> GPLGSPEFMEPLKVEKFATANRGNGLRAVTPLRPGELLFRSDPLAYTVCKGSRGVVCDRCLLGKEKLMRCSQCRVAKYCSAKCQKKAWPDHKRECKCLKSCKPRYPPDSVRLLGRVVFKLMDGAPSESEKLYSFYDLESNINKLTEDRKEGLRQLVMTFQHFMREEIQDASQLPPAFDLFEAFAKVICNSFTICNAEMQEVGVGLYPSISLLNHSCDPNCSIVFNGPHLLLRAVRDIEVGEELTICYLDMLMTSEERRKQLRDQYCFECDCFRCQTQDKDADMLTGDEQVWKEVQESLKKIEELKAHWKWEQVLAMCQAIISSNSERLPDINIYQLKVLDCAMDACINLGLLEEALFYGTRTMEPYRIFFPGSHPVRGVQVMKVGKLQLHQ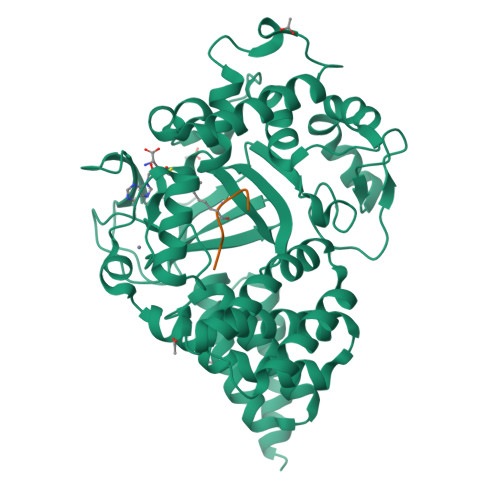GMFPQAMKNLRLAFDIMRVTHGREHSLIEDLILLLEECDANIRAS;> LKLGKSLGR>TTILSVRKGDTVVLLGDRQVTLGERIVAKSSACKLRRINDDVVIGFAGSTADAISLME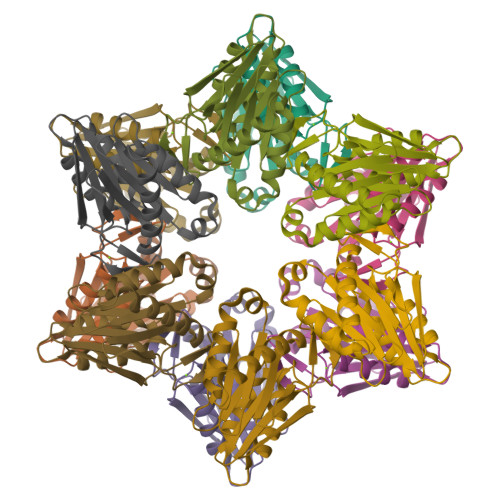KLENKIGEFPNQLTRAAVELAKEWRTDRALRRLEASLIVCSAEETLEIDGQGNVITPEADGIVAIGSGGTFAKAAARALIDVDGYDAEKIARKAMRIATDIDVFSNEHWDVEVLEHHHHHH[12x]> GLVPRGSHMWIGVISLFPEMFKAITEFGVTGRAVKHNLLKVECWNPRDFTFDKHKTVDDRPYGGGPGMLMMVQPLRDAIHTAKAAAGEGAKVIYLSPQGRKLDQGGVTELAQNQKLILVCGRYEGIDERLIQTEIDEEWSIGDYVLTGGELPAMTLIDAVARFIPGVLGKQASAEEDSFADGLLDCPHYTRPEVLEGLTVPPVLMS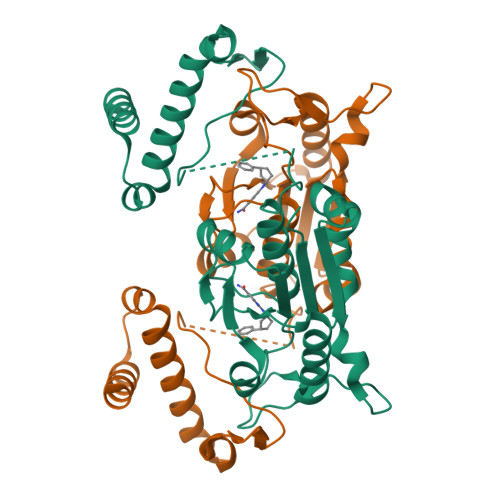GHHEEIRKWRLKQSLQRTWLRRPELLEGLALTDEQRKLLKEAQAEHNS>[4x]MSASIPDIKLSSGHLMPSIGFGCWKLANATAGEQVYQAIKAGYRLFDGAEDYGNEKEVGDGVKRAIDEGLVKREEIFLTSKLWNNYHDPKNVETALNKTLADLKVDYVDLFLIAFPIAFKFVPIEEKYPPGFYCGDGNNFVYEDVPILETWKALEKLVAAGK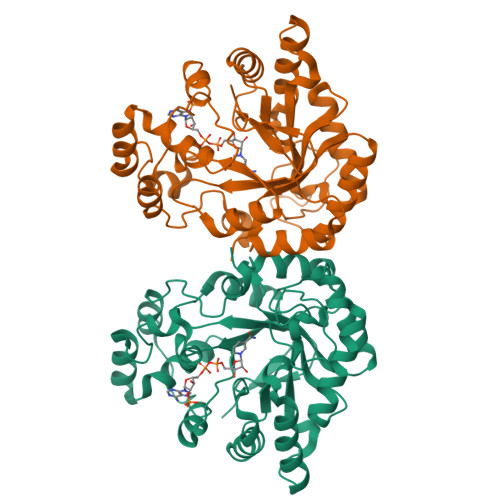IKSIGVSNFPGALLLDLLRGATIKPAVLQVEHHPYLQQPKLIEFAQKAGVTITAYSSFGPQSFVEMNQGRALNTPTLFAHDTIKAIAAKYNKTPAEVLLRWAAQRGIAVIPKSNLPERLVQNRSFNTFDLTKEDFEEIAKLDIGLRFNDPWDWDNIPIFV Protein translation relies on aminoacyl-tRNA synthetases (aaRSs) to charge tRNAs with their cognate amino acids. Plasmodium AspRS is a Class IIb aaRS that exhibits unusual sequence features compared with human AspRS, including initiation from an internal methionine, and an insert in the anticodon-binding domain. PvAspRS (96–631) was successfully crystallized as the apo protein, in complex with the natural intermediate, and with synthetic Asp-AMS and Asp-DACM, allowing insights into the binding determinants. As anticipated, PvAspRS adopts a dimeric structure with features typical of Type II aaRSs.

We solved the structure of PvAspRS with bound synthetic Asp-DACM and refined it to 2.4 Å resolution. Well-defined electron density was observed for the adduct in both chains A and B. The Asp-DACM is located in the active site pocket of the catalytic domain and interacts with a number of amino acid residues. The adenine moiety is stacked between H405 and Y409 from motif II. H405 moves from its position in the apo protein to form a parallel π stack with the adenine ring. In both chains, R396 extends to interact with the aspartate of Asp-DACM. Similarly, E398 repositions to form an H-bond with the adenine. The aspartic acid moiety of Asp-DACM also interacts with Q374, R561, and K377. Residue E352 (of the SEGG motif in Chain B) repositions to interact with the amino group of the aspartate, leading to a small movement towards the ligand. In Chain A of Asp-DACM-bound PvAspRS, two additional residues of the flipping loop (G353 and G354) are resolved compared with the apo protein.

>[2x]AERENLKNEATKVLEHVCEDINKESYGFVKISKMKENEKEIRLFNLEEIYHSLMKVGGSGATDGGKREDDAASHSVVAESNGAHLLQSDIWVRGRIHDIRSKGSLAFIILRHKLYSMQCILDIKHNDNDKNMMKWVSNLPLESIVDIKGKLSKPEVPIDSTNIKYEAHIRKIFCISKTAKELPFLLKDANMKETNEEGSIKVNQDNRLNNRCVDLRTYANYSIFCLQSQICTIFKNFLLENNFIEIHTPKLLGESSEGGANAFQINYFNQKGFLAQSPQLYKQMCINSGFDRVFEVAPVFRAENSNTYRHLCEYVSLDVEMTYKYDYLENVHFYDSMFKHIFTELSKGGKNEMLIKTVKGQYPCEDFQWLEETPIFTYEEAIKMLIQHGKLHLKEEEILAYDMSTDMEKELGKIVKASHHTDYYIIINFPSALRPFYTMYKEDEPAISNSYDFFMRGEEILSGSQRISDVNLLLENIKRFNLDANKLNFYIDSFAYSSYPHSGCGIGLERVLMLFLGLNNIRKTSLFPRDPKRLIP>MVERLLEIIERSLRKCPWLEKQSIETLLEALASEIEEVAEAVKKNDLANLEEEIGDMIYDALLVAAVAQRDYGIDLESAI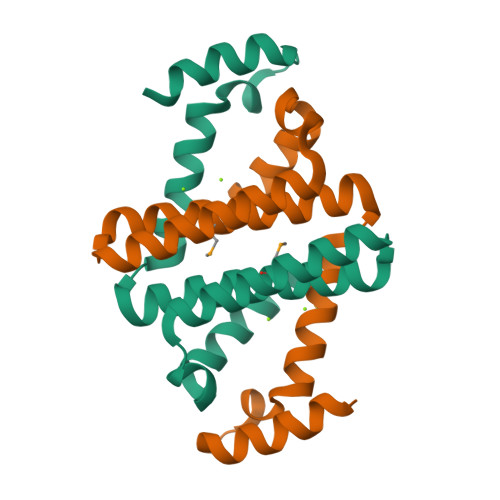QKVVEKISHRKPWLFWEEKISLEEAEKIWKERKKKI[2x]>MSLLKQKILNRESGIITYGITPPKKNNTEEKIKEISQKHIERISGLDIDGLVIYDLQDEKERVSEERPFPFIETIDPQIYSENYLKDLKIPKIIYRCVGKYTPDEFRRLTRPVSGQDAFSVFVGAASRNQSVLLKLSDAYKIRQDVNPDLLLGGVAIPERHMKNTDEHLRIIDKINKGCKYFITQAVYNVEAAKDFLSDYYYYSKNNNLKMVPIIFTLTPCGSTKT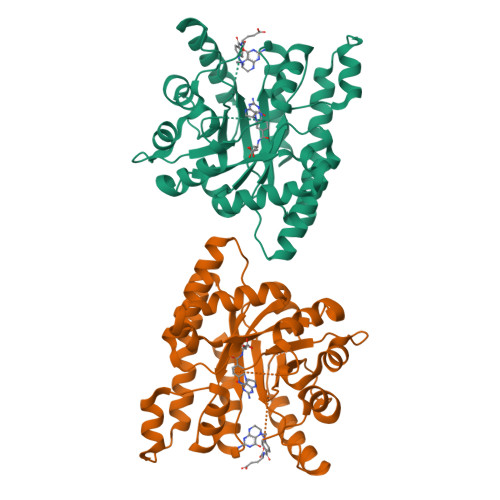LEFMKWLGISIPRWLENDLMNCEDILNKSVSLSKSIFNELMEFCLEKGIPIGCNIESVSVRKVEIEASIALAKDIKYIMKGEGHHHHHH[2x]DHAR catalyses the reduction of DHA to AsA using glutathione (GSH) as a hydrogen donor before the spontaneous hydrolysis of DHA to irreversibly form 2,3-diketogulonic acid. To expand our knowledge of the underlying molecular mechanism of OsDHAR activity against ROS, high-resolution crystal structures of the apo-form, AsA-bound, and GSH-bound OsDHAR were examined at 1.9, 1.7, and 1.7 Å resolution, respectively. The structure shows that the asymmetric unit contains one molecule of OsDHAR and adopted a canonical GST fold, consisting of three β-strands and three α-helices in the N-terminal subdomain (residues 4–84) and six α-helices in the C-terminal subdomain (residues 94–210), although OsDHAR showed modest sequence identity (~20%) with GSTs. Structural comparison studies revealed that Cys20 is a catalytic residue and that Lys8 directly interacts with AsA and GSH to reduce Cys20.

Here, we present the first crystal structure of OsDHAR. Most of the residues were well-resolved, except for the N-terminal methionine residue. Notably, OsDHAR was found to be a monomer under both reducing and oxidizing (10 mM H2O2) conditions. After inspection of the apo-OsDHAR structure, we predicted that the highly conserved Cys20 residue acts as the catalytic nucleophile and found that this residue is located at the cleft between the N- and C-terminal subdomains. In the apo-OsDHAR structure, the OG atom of Ser23 is 3.4 Å away from the SG atom of Cys20, which is an acceptable hydrogen bonding distance considering the rotational movement of the side chains of Ser23 and Cys20. Notably, the three-dimensional structure indicates that OsDHAR contains a broad, uncharged cleft between the α2-helix and the α3-helix as the putative binding site for non-native protein folding intermediates for its chaperone-like activity.

> MHHHHHHASENLYFQGAMGVEVCVKAAVGHPDTLGDCPFSQRVLLTLEEKKVPYEMKLIDVQNKPDWFLKISPEGKVPVFNGGDGKWIPDSDVITQVIEEKYPTPSLVTPPEYASVGSKIFSCFTTFLKSKDPNDGSEKALLTELQALEEHLKAHGPFINGQNISAADLSLAPKLYHLQVALEHFKGWKIPEDLTNVHAYTEALFSRESFIKTKAAKEHLIAGWAPKVNA>MGHHHHHHVSSTNGFSATRSTVIQLLNNISTKREVEQYLKYFTSVSQQQFAVIKVGGAIISDNLHELASCLAFLYHVGLYPIVLHGTGPQVNGRLEAQGIEPDYIDGIRITDEHTMAVVRKCFLEQNLKLVTALEQLGVRARPITSGVFTADYLDKDKYKLVGNIKSVTKEPIEASIKAGALPILTSLAETAS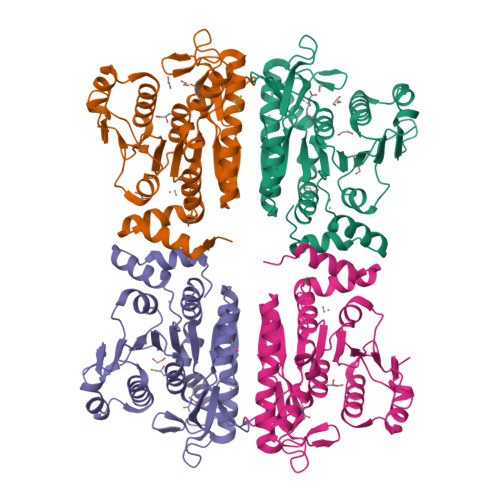GQMLNVNADVAAGELARVFEPLKIVYLNEKGGIINGSTGEKISMINLDEEYDDLMKQSWVKYGTKLKIREIKELLDYLPRSSSVAIINVQDLQKELFTDSGAGTMIRRGYKLVK[4x]>[2x]MRSRRVDVMDVM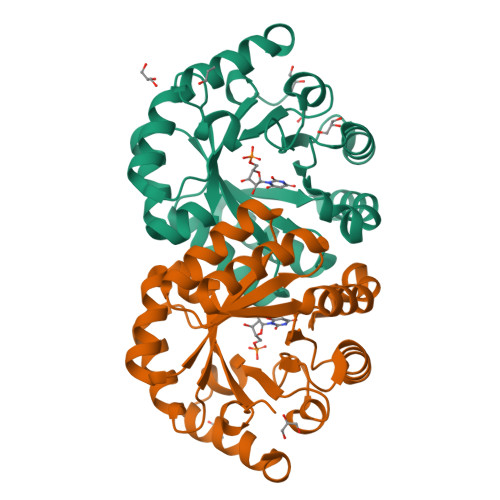NRLILAMDLMNRDDALRVTGEVREYIDTVKIGYPLVLSEGMDIIAEFRKRFGCRIIADFKVADIPETNEKICRATFKAGADAIIVHGFPGADSVRACLNVAEEMGREVFLLTEMSHPGAEMFIQGAADEIARMGVDLGVKNYVGPSSRPERLSRLREIIGQDSFLISPGVGAQGGDPGETLRFADAIIVGRSIYLADNPAAAAAGIIESIKDLLNP>[2x]MSQPLTTNSVLVEEAAADGDSSAAAPPLFDYHRIDQKLLQNIVYDALVWSTLNCLLVGDKSVQRSGRVPGVGLVHLPLSLLPGPFPESHWKQGCELAPIFNELVDRVSLDGKFLQESLSRTKNADEFTSRLLDIHSKMLQINKKEDIRMGIVRSDYMIDEKTKSLLQIEMNTISTSFALIGCLMTGLHKSLLS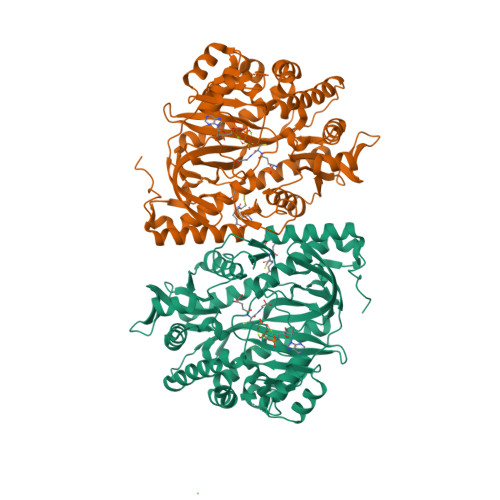QYGKFLGLNSNRVPANNAVDQSAEALAKAWSEYNNPRAAILVVVQVEERNMYEQHYISALLREKHHIRSIRKTLTEIDQEGKILPDGTLSVDGQAISVVYFRAGYTPKDYPSESEWRARLLMEQSSAIKCPTISYHLVGTKKIQQELAKPGVLERFVENKDHIAKLRACFAGLWSLEDSDIVKKAIENPELFVMKPQREGGGNNIYGDELRETLLKLQEAGSQEDAAYILMQRIFPATSPAILVRDGNWDTGHVISEAGIFGTYLRNKDKIIINNESGYMVRTKISSSYEGGVLPGFGVVDTVYLT> MTVTTTYPGVYLSEDAVSSFSVNSAATAVPLFAYDSENTNTINKPIQVFRNWAEFTVEYPTPLEDAFYTSLSLWFMHGGGKCYLVNEANIADAVAQYDDITLIVAAGTDTTTYTAFTTVVGQGYRIFGLFDGPKEKIAGTAKPDEVMEEYPTSPFGAVFYPWGTLASGAAVPPSAIAAASITQTDRTRGVWKAPANQAVNGVTPAFA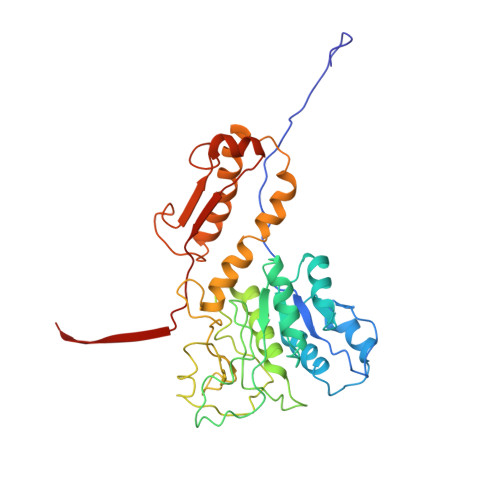VSDDFQGKYNQGKALNMIRTFSGQGTVVWGARTLEDSDNWRYIPVRRLFNAVERDIQKSLNKLVFEPNSQPTWQRVKAAVDSYLHSLWQQGALAGNTPADAWFVQVGKDLTMTQEEINQGKMIIKIGLAAVRPAEFIILQFSQDIAQ>[12x]HMSTSISEAEPPRVLITGGLGQLGVGLANLLRKRFGKDNVILSDIRKPPAHVFHSGPFVYANILDYKSLREIVVNHRISWLFHYSALLSAVGEANVSLARDVNITGLHNVLDVAAEYNVRL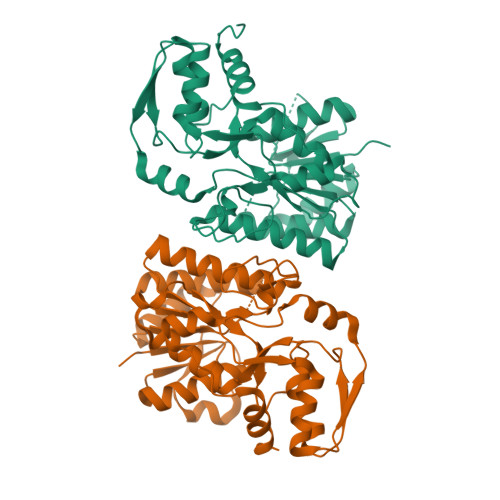FVPSTIGAFGPTSPRNPAPDLCIQRPRTIYGVSKVHTELMGEYYYYRYGLDFRCLRYPGIISADSQPGGGTTDYAVQIFHAAAKNGTFECNLEAGTRLPMMYISDCLRATLEVMEAPAERLSMRTYNISAMSFTPEELAQALRKHAPDFQITYCVDPLRQAIAESWPMILDDSNARKDWGWKHDFDLPELVATMLNFHGVSTRVAQVN Proteins that contain the DUF2874 domain constitute a new Pfam family PF11396. Members of this family have predominantly been identified in microbes found in the human gut and oral cavity. Sequence analysis and structural comparisons reveal that BVU2987 and other DUF2874 proteins are related to β-lactamase inhibitor protein, PepSY and SmpA_OmlA proteins and hence are likely to function as inhibitory proteins. Analysis of our structure and of the available sequences shows that collectively this family forms part of a larger superfamily of bacterial periplasmic proteins that all adopt a fold similar to β-lactamase inhibitor protein (BLIP-like fold) and appear to share some broad spectrum of inhibitory function.

BVU2987 is a 145-residue protein with a calculated pI of 5.36 and is annotated as a putative periplasmic protein based on the predicted N-­terminal signal peptide. The structure of BVU2987 was determined by MAD phasing to 1.85 Å resolution. The crystallized protein contained residues 20–145 of the full-length protein and an N-terminal glycine (that remained after the cleavage of the expression and purification tag). The final model contained one monomer, one cacodylate anion (from the crystallization condition) and 133 water molecules in the asymmetric unit. Crystal-packing analysis using PISA, in addition to analytical size-exclusion chromatography coupled with static light scattering, indicated that the monomer was the favored oligomeric form in solution. The monomer is formed by a tandem repeat of a structural motif, possibly arising from a gene-duplication event, comprised of four antiparallel β-strands and a short helix–loop–long helix. Thus, residues 28–85 and 92–145 can be superimposed with an r.m.s.d. of 1.7 Å and a sequence identity of 22% over 54 aligned Cα atoms. Although these aromatic residues are not conserved in BVU2987, other aromatic residues (Trp57, Phe58, Tyr122, Trp130 and Phe138) are present in the corresponding shorter loops in BVU2987, which may be functionally important. For BVU2987, the negatively charged concave surface is most likely to reflect binding to a positively charged partner. The BVU2987 structure is the first structural representative of a novel protein family, which has now been added to the Pfam database as DUF2874.

> GADDDKPIQVNQLPQTAQTFIKTHFPDNKVAMAKMETDWFDKSYDVIFTNGDKLEFDKKGIWTEVNCKYSAVPVAVVPDAIKKYVATNYPDAKMLKIERDKHDYEVKLSNGWEIKFDMQFNVIDIDN The HAstV capsid precursor protein comprises several domains, including a highly basic amino terminus that binds to the RNA genome, a core domain that forms the icosahedral shell, a spike domain that forms dimeric protrusions, and an acidic domain with unknown function at the carboxy terminus. The HAstV-VA1 spike forms a dimer and shares a core beta-barrel structure with other astrovirus capsid spikes but is otherwise strikingly different, suggesting that HAstV-VA1 may utilize a different cell receptor, and an infection competition assay supports this hypothesis. The HAstV-VA1 spike structural domain forms a homodimer, with each protomer encompassing residues 408–684. Also similar to other HAstV spikes, the structural domain of each protomer of the HAstV-VA1 spike comprises a core antiparallel beta-barrel, formed by beta-strands 1, 9, 10, 16, and 18.

We began by studying the capsid sequence from the first neuronal HAstV-VA1 (HAstV-VA1neuro) found to be associated with encephalitis in an immunocompromised patient who ultimately died after 71 days of hospitalization. In a different approach, we generated a larger construct encoding the C-terminal residues 394–758 of the HAstV-VA1neuro capsid protein (~43 kD), and expressed this protein in Sf9 insect cells. Despite low yields (micrograms per Liter), this recombinant protein was soluble, and limited proteolysis with trypsin resulted in a trypsin-resistant fragment of ~36 kD. Mass spectrometry analysis revealed a mass of 36,020 Daltons, similar to a predicted tryptic fragment of 35,970 Daltons that would be generated by cleavage after arginine 697. Thus, a new construct encoding the HAstV-VA1neuro capsid residues 394–697 (~36 kD) was generated as a fusion protein with superfolder GFP (sf-GFP) and expressed in insect cells with improved yields (milligrams per Liter). Following removal of the sf-GFP, the HAstV-VA1neuro capsid spike protein was crystallized and diffraction data to a resolution of 2.73 Å was collected. The structure of the HAstV-VA1neuro capsid spike was solved to 2.73 Å resolution. Finally, to evaluate if there are structural changes in the spike that drive infection of the CNS, we aligned the HAstV-VA1gastro and HAstV-VA1neuro spike structures, which resulted in an RMSD of 0.78 Å and TM-score of 0.97, revealing that no major structural differences are observed. Specifically, only six variable sites were observed in HAstV-VA1gastro spike sequences, whereas 27 variable sites were observed in HAstV-VA1neuro spike sequences. Statistical analyses confirm that there is a significant decrease in antibody binding to the HAstV-VA1neuro spike compared to the HAstV-VA1gastro spike. Thus, these data reveal that mutations present in the HAstV-VA1neuro spike protein result in reduced anti-HAstV-VA1gastro polyclonal antibody binding.

>[2x]NTTIESIGNNNQQWPIPLTGVPVGDFYVYGRMTTLHMGGQSGIQATTLVNGMIYRTDHPEPSTSPVSNWEFTVLENNTIVGAGMGCVWFQKSEVLVWTLDGQKLSGWNTLDGVGTTQLTVAWRQHNRTIYGWANVVAWNSEEWHTNAERLHQPTLRLTYWLVKINVSSEPEDFDVVQKFPLAYLEDYTTAQSKSAIQKLNFQTFQKPEGGGTLRAQYSTVPRQGDFAVIWQIGRHNFDMSTGKGTPVESLSDYVMPEQKDARIGMWYRALTSVGPRSDMLTLHFHFPTVEKDLVEQIIDQIQHR>[2x]GSVLQKEGIEISEGTGYDLSKEPGAATVKALEQGTIVISYKTTSENAIQSLLSVGNGTKGNQDRHFHLYITNAGGVGMELRNTDGEFKYTLDCPAAVRGSYKGERVSNT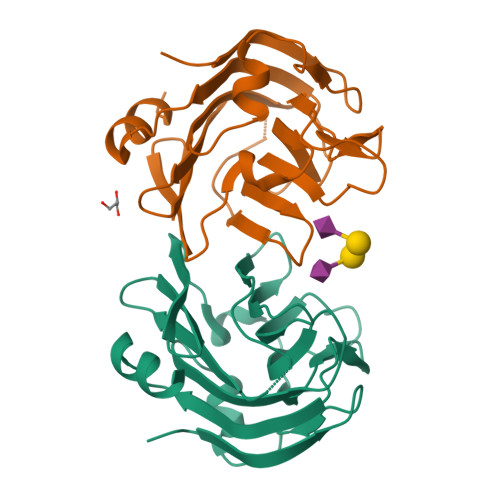VALKADKENKQYKLFANGELIATLDQEAFKFISDITGVDNVMLGGTMRQGTVAYPFGGSIERMQVYRDVLSDDELIAVTGI>WSHPQFEKGAETAVPNSEDVMKRAQGLFKPIPAKPPVMKDNPASPSRVELGRMLFFDPRLSASHLISC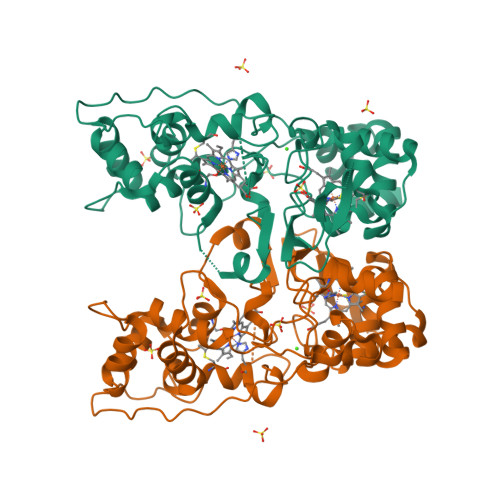NTCHNVGLGGTDILETSIGGGWQKGPRNSPTVLNAVYNIAQFWDGRAEDLAAQAKGPVQASVEMNNKPENLVATLKSIPGYPPLFRKAFPGQGDPVTFDNVAKAIEVFEATLVTPDAPFDKYLKGNRKAISSTAEQGLALFLDKGCAACHSGVNMGGTGYFPFGVREDPGPVVRPVDDTGRYKVTSTAADKYVFRSPSLRNVAITMPYFHSGKVWKLKDAVKIMGSAQLGISITDADADKIVTFLNTLTGAQPKVMHPVLPPNSDDTPRPVSN[2x]> MSKILV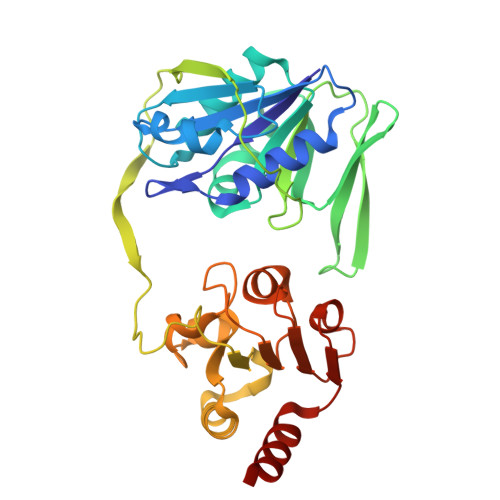IAEHRRNDLRPVSLELIGAANGLKKSGEDKVVVAVIGSQADAFVPALSVNGVDELVVVKGSSIDFDPDVFEASVSALIAAHNPSVVLLPHSVDSLGYASSLASKTGYGFATDVYIVEYQGDELVATRGGYNQKVNVEVDFPGKSTVVLTIRPSVFKPLEGAGSPVVSNVDAPSVQSRSQNKDYVEVGGGNDIDITTVDFIMSIGRGIGEETNVEQFRELADEAGATLCCSAPIADAGWLPKSRQVGQSGKVVGSCKLYVAMGISGSIQHMAGMKHVPTIIAVNTDPGASIFTIAKYGIVADIFDIEEELKAQLAA> MEPQREFFHIAGRSAKEYLSENLVQFIQATQNYFNIGEKFRDPYVAPSAGVTTDRSQKLQLRVVPIQTEDNVNYYKARFTLNVGDNRLVDLGSSYFDIKGTLDRGPSFKPYGGTAYNPLAPKSAPINSAFTVGNDTHFVAQLPQTYAAGGTGVTEAIQQQVSGVDPNPQVGQPNYAGPVVVNTTNNAGLGRIVSADSEGQQFPCYGAYAPPQSAGGDVSTAAVTKTYINTTNNNGRVSGTMATDTITWENPDAHFADFVDDRRATAAGNRPNYIGFRDNFIGMMYYNSGSNTGSFSSQTQQLNIVLDLNDRNSELSYQYLLADLTSRWHYFALWNQAVDDYDHHVRILENDGYEEGPPNLAFPPHVISNPFAPAAVGTGMTVNEQQQTAAVTANTVALIGYGNIPAVEMNLPANLKRTFLYSNVAMYLPDTYKFTPANVDLPENHLSYGYINGRLPLPNIVDTWTDIGARWSLDVMDTVNPFNHHRNTGLKYRSQLLGNGRYCDFHIQVPQKFFAIKNLLLLPGTYNYEWYFRKDPNMVLQSTLGNDLR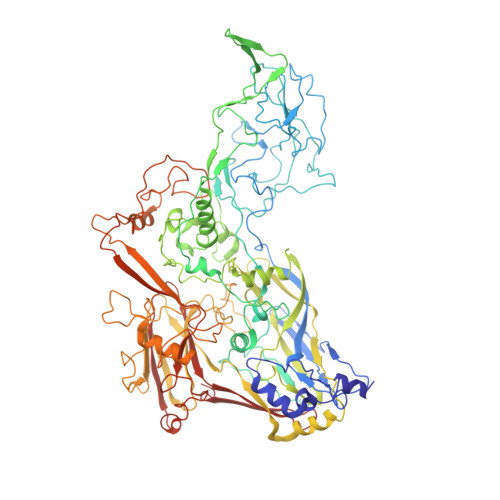ADGASITYTQINLYVSFFPMNYDTQSELELMLRNATNDQNFSDYLGAVNNLYQIPAGSSTVVVNIPDRSWGAFRGWSFTRLKVSETPRIGATQDPNFQYSGSIPYLDGTFYLSHTFQRCSIQWDSSVPWPGNDRMLTPNWFEIKRPINQDAEGNDTMQSNLTKDFFMVQMAASYNQGYQGFNWPNCTKHYGFINNFEPMSRQVPEYGANYPNLMAAYLANPQTMPIWNNCGFQQKTATNVLLERCGHPYVANWPYPLSGRNAVPNQVTERKFLVDRYLWQIPFSSNFLNMGTLTDLGQNVMYANSSHSLNMQFTVDPMTEPTYLMLLFGVFDQVVINQPTRSGISVAYLRLPFASGSAAT> MPQDVRFDLPFDTPVSEHLEYARARHLRWVWEMRLVRSRDGFEEYKSWDLPQAAARTYPHASADDMVVLMNWFSLAFLFDDQFDASRPDRADRIAEVARELIVTPLRPAGSPPRVACPITLAWAEVWKYLSHGMSLTWQTRFAASWGRFLVAHCEEVDLAARGLEGTLGLDEYAEFRRRTVGIHHSIDAGERSRGFEVPAQAMGHPVMERMRDLAADTIGFMNDIHSFEREKRRGDGHNLIAVLRRERGCSWQQATDEAYRMTIACLDEYLEL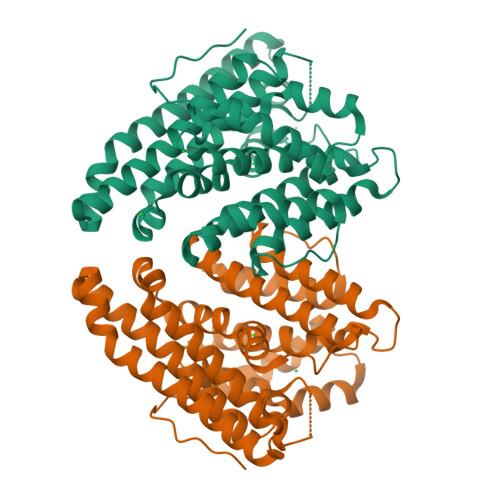QERVPQMCDELRLDEAERDRVRMGVEAIQHWINGNYEWALTSGRYAAAKEGPVATAELAGRGSVDDLLTV> SQNKSYPSCILPNNNRHQIFNTTQGHYDAVSFIYIPIDGGYMSGSGVVVGENEILTNKHVVNGAKGNPRNISVHPSAKNEN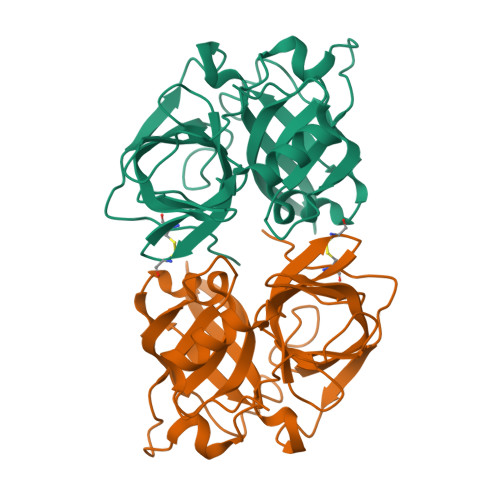DYPNGKFVGQEIIPYPGNSDLAILRVSPNEHNQHIGQVVKPATISSNTDTRINENITVTGYPGDKPLATMWESVGKVVYIGGEELRYDLSTVGGNSGSPVFNGKNQVIGIHYGGVCNKYNSSVYINDFVQQFLRNNIPDINIQ>[6x]NTANLVRKEGFGAAVRSSIEELADWAEVERPDLARVTPDGRVVILFTDIEESTALNERIGDRAWVKLISSHDKL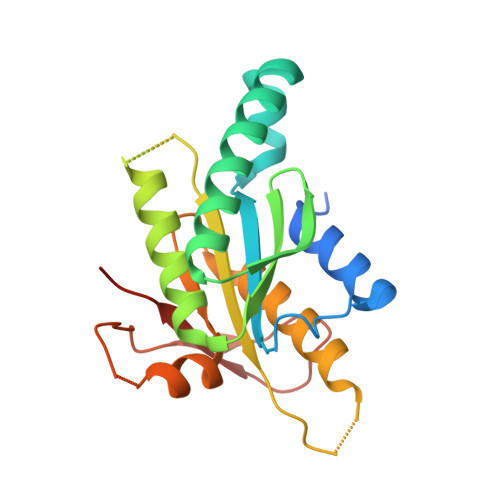VSDLVRRQSGHVVKSQGDGFMVAFARPEQAVRCGIELQRALRRNANRKRHEEIRVRIGIHMGRSVRRGDDLFGRNVAMAARVAAQAAGGEILVSQPVRDALSRSDGIRFDDGREVELKGFSGTYRLFAVLASPDPG> SNAMSSESDAANTEPEVLVEQRDRILIITINRPKAKNAVNAAVSRGLADAMDQLDGDAGLSVAILTGGGGSFCAGMDLKAFARGENVVVEGRGLGFTERPPTKPLIAAVEGYALAGGTELALAADLIVAARDSAFGIPEVKRGLVAGGGGLLRLPERIPYAIAMELALTGDNLPAERAHELGLVNVLAEPGTALDAAIALAEKIT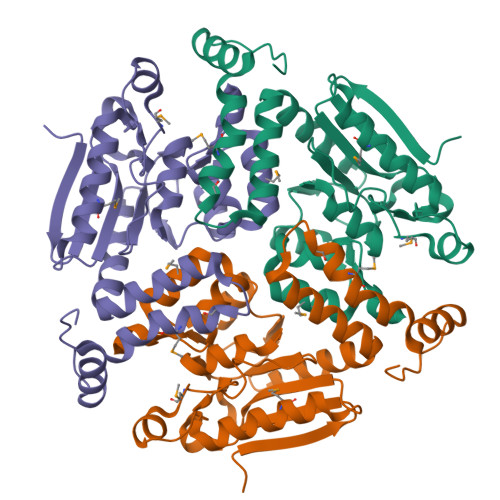ANGPLAVVATKRIITESRGWSPDTMFAEQMKILVPVFTSNDAKEGAIAFAERRRPRWTGT2-({2-[(6-chloro-1,2,3,4-tetrahydroacridin-9-yl)amino]ethyl}amino)-5-hydroxynaphthalene-1,4-dione | C25 H22 Cl N3 O3 | 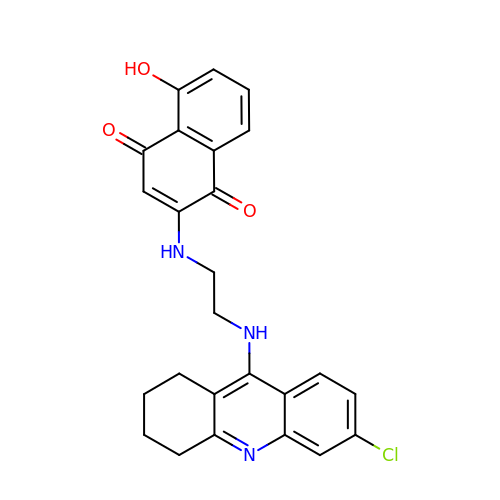QOYHHKMVCBONOU-UHFFFAOYSA-N> MGSKYSKATNSINDALSSSYLVPFESYRVPLVDLEEATNNFDHKFLIGHGVFGKVYKGVLRDGAKVALKRRTPESSQGIEEFETEIETLSFCRHPHLVSLIGFCDERNEMILIYKYMENGNLKRHLYGSDLPTMSMSWEQRLEICIGAARGLHYLHTRAIIHRDVKSINILLDENFVPKITDFGISKKGTELGQTHLSTVVKGTLGYIDPEYFIKGRLTEKSDVYSFGVVLFEVLCARSAIVQSLPREMVNLAEWAVESHNNGQLEQIVDPNLADKIRPESLRKFGDTAVKCLALSSEDRP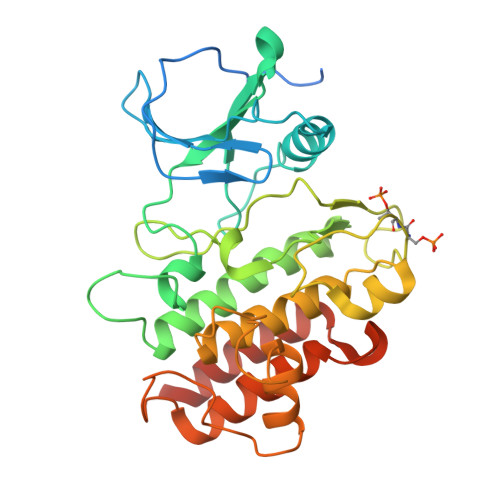SMGDVLWKLEYALRLQESVIHHHHHH Pif1 is a DNA helicase belonging to family SF1B of Superfamily 1 (SF1), which unwinds dsDNA with 5′ to 3′ directionality. Pif1 is involved in DNA repair and is necessary for the maintenance of mitochondrial and nuclear genomes integrity, in the regulation of telomerase activity and in the replication fork progression. We were able to crystallize the helicase core of Pif1 from the thermophilic bacteria Deferribacter desulfuricans and Sulfurihydrogenibium sp., which are moderate thermophilic bacteria, living at an average temperature of 65 °C. Pif1 from these bacteria are named DdPif1 and SsPif1, respectively. The helicase core of Pif1 from thermophilic bacteria is very similar to other bacterial Pif1 structures already solved. The HC contains the features of previously described SF1B helicases: two RecA-like domains 1A and 2A containing insertions 1B and 2B, respectively.

DdPif1 apo crystallized in spacegroup C2221 with one molecule in the asymmetric unit and DdPif1 in the complex with the nucleotide analogue AMPPNP crystallized in spacegroup P21212 with two molecules in the asymmetric unit. Only DdPif1 was solved in two different states, apo and in complex with the ATP analogue AMPPNP. Structural changes upon nucleotide binding are moderate in the absence of ssDNA, as already observed for BsPif1 and ToPif1. The main difference is the folding of the N-terminal part of DdPif1 (residues 1-20). This N-terminal part is not visible in the DdPif1 structure and may be disordered. Since we observed that the N-terminal part is not visible in the DdPif1 apo structure and contributes to nucleotide binding, we hypothesized that it could flexible. Therefore, we analysed the structural changes of DdPif1 apo in solution by small-angles X-ray scattering (SAXS). The molecular weight of DdPif1, estimated from I, Porod volume, and Volume of correlation (Vc) is 50 kD, which is consistent with a monomer of DdPif1 in solution. Thus, the DdPif1-apo structure was modelled by flexible fitting with DADIMODO by introducing flexibility in the N-terminal tail (residues 1-20) and the linker between 1A and 2A domains. Therefore, in the absence of a nucleotide, the N-terminal may be unstructured and becomes folded upon nucleotide binding.

> MKLALNTEFKKAIDLATNSSKNLFITGKAGTGKSTFLKYLINELLFDAVVLAPTGVAAINIGGETIHSFFNFPINITPDKIPDLFIYDYEIYKYVNTIIIDEISMVRADLLDCIDLFLKRVKNPKLPFGGTKMIFIGDLYQLPPVLTNHQKKAFNMEYESPYFFSAKVFKEMDMEFIEFETIYRQSDKLFIDILNRIRNNTVTDEDIKIINSRVQDKIDNDDGYIYITTVNKKAEEINNQKLDKLKGKLYKLNGTLKGNFDENSLPTPKNLHLKIGAQVMLLNNAPDRMWVNGTIGTITNIFPDEMIIELALENGNIVEITPFKWDMIKFTYDKKEKKMLSETIGSYTQFPLKLAYAITVHKSQGKTFHKVIIDTSRHFFAPGQFYVALSRCTSLDGIILTKKITKNSIILDKKVVNFLTNFQYQLSEKKTPLEEKISILKRAIERNSPLEIVYLKTKDEKSKRVIIPKEVGEMVYSGKSFMGLKGFCTMRNDERVFRIDRILEIKEIND>MSTGDFLTKGIELVQKAIDLDTATQYEEAYTAYYNGLDYLMLALKYEKNPKSKDLIRAKFTEYLNRAEQLKKHLESEEANAAKKSPSAGSGSNGGNKKISQEEGEDNGGEDNKKLRGALSSAILSEKPNVKWEDVAGLEGAKEALKEAVILPVKFPHLFKGNRKPTSGILLYGPPGTGKSYLAKAVATEANSTFFSVSSSDLVSKWMGESEKLVKQLFAMARENKPSIIFIDQVDALTGTRGEGESEASRRIKTELLVQMNGVGNDSQGVLVLGATNIPWQLDSAIRRRFERRIYIPLPDLAARTTMFEINVGDTPCVLTKEDYRTLGAMTEGYSGSDIAVVVKDALMQPIRKIQSATHFKDVSTEDDETRKLTPCSPGDDGAIEMSWTDIEADELKEPDLTIKDFLKAIKSTRPTVNEDDLLKQEQFTRDFGQEGN[6x];>MASNAARVVATAKDFDKVGLGIIGYYLQLYAVELILSEEDRSQEMTALATELLDTIEAFKKEIGGESEAEDSDKSLHVMNTLIHDQEKAKIYMLNFTMSLYNEKLKQLKDGPWDVMLKRSLWCCIDLFSCILHLWKENISETSTNSLQKRIKYCKIYLSKLAKGEIGSSDEKTLDYADFADDSEEIKDEDVDHQTSDLENNNNDKVEGLAPKDQTTSYEPVDEVPEFIDDADSVNEEEQTVDKNEDAITKDEQQVVKKEVDLTRPSAPSEPAAAEHKSYTKDELTKIMDRASKIEQIQKLAKYAISALNYEDLPTAKDELTKALDLLNSI[8x]

The disassembly of ESCRT-III is mainly mediated by the Vps4 protein that is a member of the type I AAA+ ATPase (ATPase associated with various cellular activities) family and oligomerizes into a functional hexamer with elevated ATPase activity upon binding to ATP6. Powered by ATP hydrolysis, the Vps4 oligomer, promoted by the cofactor protein Vta1 (Vps twenty associated 1), disassembles ESCRT-III polymers into individual ESCRT-III subunits available for recycling. Vps4 protein contains an MIT (microtubule interacting and trafficking) domain at the N terminus, a single ATPase cassette comprising a large ATPase domain and a small ATPase domain with a β-domain inserted within it, and a C-terminal helix8111213. In this study, using Vps4 from yeast, we solved the structures of the ATP-bound Vps4E233Q hexamer at 3.9 Å resolution and its complex with Vta1 at 4.2 Å resolution, both determined by single-particle electron cryo-microscopy (cryo-EM) without any symmetry imposed.

We obtained 3D reconstruction of the Vta1-bound Vps4E233Q hexameric complex at a resolution of 4.2 Å. The structure of the ATP-bound Vps4E233Q–Vta1 complex also contains a hexameric ring of the Vps4E233Q similar to that of the Vta1-free Vps4E233Q hexamer. After docking the Vps4E233Q hexamer into the EM map, we can still observe some clear extra densities located between neighbouring Vps4E233Q subunits of subunit B to F distributed at the periphery of the ring. We attributed these densities to the Vta1 protein. We were able to build an atomic model for the six Vps4E233Q molecules and four Vta1 CTD dimers in the cryo-EM map of the ATP-bound Vps4E233Q–Vta1 complex. The overall structure of the Vta1-bound Vps4E233Q hexamer and the Vta1-free Vps4E233Q hexamer share similar conformations with a root mean square deviation (r.m.s.d.) of 2.18 Å overall Cα atoms. The structure features of the Vta1-free Vps4E233Q hexamer described above, including the loose contact between subunit A and its neighbouring subunits, the spiral arrangement of subunits from A through F and the different conformation of subunit A compared with other subunits, are all preserved in the Vta1-bound Vps4E233Q hexamer, suggesting that Vta1 binding does not, or at least not significantly, alter the conformation of the ATP-bound Vps4E233Q hexamer. The interface of the two CTDs in one CTD dimer is roughly perpendicular to the Vps4E233Q hexameric ring, resulting in one CTD, referred to as inner CTD, closer to the ring centre than the other one, referred to as outer CTD. Vta1 CTD dimer bridges between two adjacent Vps4E233Q subunits in two different modes. One mode is guided by the interactions of the β-domain and helixes α7 and α9 of the small ATPase domain from one Vps4E233Q subunit with the regions around the tip of α8/α9 helix hairpin from the outer CTD of one CTD dimer and the N-terminal half part of the helix α8 from the inner CTD of the same dimer, respectively.> GHMMVKIMPNLPGLYFLQ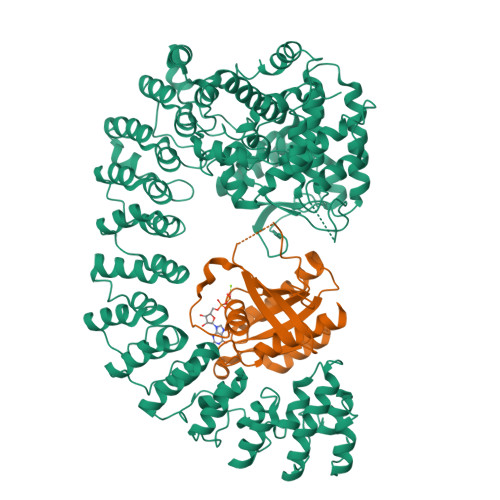AYPSEEIWRLFVDGRFWSKENGWRGYESREPGSLNAALESLCSIALQVEKSGEEFELSVDLIKRIHKKSGKKVEELQEKNPGELRTDEPVSFCIPAGRASIKGIEEFLSLVFLTEGGAEFGPGKAGPFGPRFDKNYFKNLNPEQIPDLAKQIYFDMSKYGHSNTNHFYLAVMKNVDVYLEKITQSYNKEIKTAETLDEKLKIIVKHIRMYEVLHPFRDANGRTFVNNLLNILLMQQGLPPATFYEPNVFDLYSAEELVVVVKEAIFNTVEIIEQSKRKTPITLYGYHSSLEEQTKFRDMLDSPSYEKIKHMDFSDLNPEKLHLKTQKCLSSLNEQYPLHRGAIYLSDPGEIKLLLSNRNESQINQQIEQGAPPIYVGKTPAHLAVISGNMAMLDELIAKKADLSLQDYDGKTALHYAAECGNMQIMGKILKVVLSQEDAIKVLNIKDNHGKTAFHYAAEFGTPELISALTTTEVIQINEPDNSGSSAITLAYKNHKLKIFDELLNSGADISDELLDAIWARKDKETLGKIIAKNEKILLNKEAFRIAISLGSVSLVKKFLRAGVDIDIPLTKDKATPLMLSINSGNPKLVSYLLKKGANTRLTDTSGNSVLHYVFYSKAENREALANIITEKDKKLINQPNANGNPPLYNAVVVNDLKMATILLEMGARVDFEDRLGNNILHSAMRRCDLPIILDIVKKDSTLLHKRNSERRNPFHQALHEMHTFPSSKETEEIHFMNLSDLLLKEGVDLNKKDIKGKTILDIALSKQYFHLCVKLMKAGAHTNI;> GPMPEYDYLFKLLLIGDSGVGKSCLLLRFADDTYTESYISTIGVDFKIRTIELDGKTIKLQIWDTAGQERFRTITSSYYRGAHGIIVVYDVTDQESYANVKQWLQEIDRYASENVNKLLVGNKSDLTTKKVVDNTTAKEFADSLGIPFLETSAKNATNVEQAFMTMAAEIKKRMG> HNFLRREIKIEGDLVLGGLFPINEKGTGTEECGRINEDRGIQRLEAMLFAIDEINKDDYLLPGVKLGVHILDTCSRDTYALEQSLEFVRASLTKVDEAEYMCPDGSYAIQENIPLLIAGVIGGSYSSVSIQVANLLRLFQIPQISYASTSAKLSDKSRYDYFARTVPPDFYQAKAMAEILRFFNWTYVSTVASEGDYGETGIEAFEQEARLRNISIATAEKVGRSNIRKSYDSVIRELLQKPNARVVVLFMRSDDSRELIAAASRANASFTWVASDGWGAQESIIKGSEHVAYGAITLELASQPVRQFDRY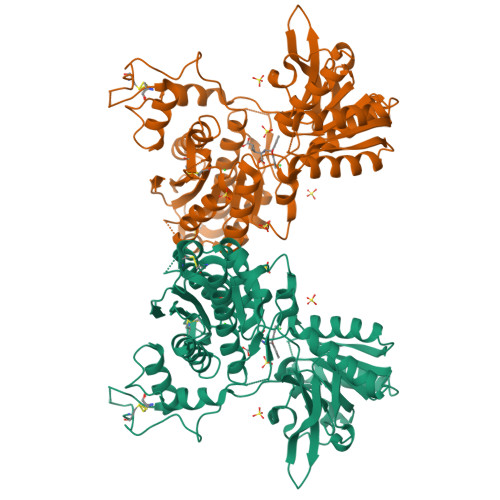FQSLNPYNNHRNPWFRDFWEQKFQCSLQNKRNHRRVCDKHLAIDSSNYEQESKIMFVVNAVYAMAHALHKMQRTLCPNTTKLCDAMKILDGKKLYKDYLLKINFTAPFNPNKDADSIVKFDTFGDGMGRYNVFNFQNVGGKYSYLKVGHWAETLSLDVNSIHWSRNSV> SMADLLVPKLTASVTDGAVGVTVDAPVSVTAADGVLAAVTMVNDNGRPVAGRLSPDGLRWSTTEQLGYNRRYTLNATALGLGGAATRQLTFQTSSPAHLTMPYVMPGDGEVVGVGEPVAIRFDENIADRGAAEKAIKITTNPPVEGAFYWLNNREVRWRPEHFWKPGTAVDVAVNTYGVDLGEGMFGEDNVQTHFTIG

The transpeptidase LtdMt2 catalyzes the formation of the (3–3) cross-links characteristic of the peptidoglycan layer in the Mycobacterium tuberculosis cell wall. The structure analysis reveals that LdtMt2 folds into three domains: two domains in the N-terminal part, both of which show an immunoglobulin-related fold, and a C-­terminal transpeptidase domain. Combining the structures of the two fragments provides a view of the complete three-domain extramembrane part of LdtMt2 and shows that the protein extends at least 80–100 Å from the plasma membrane into the peptidoglycan layer and thus defines the maximal distance at which cross-links are formed by this enzyme. LdtMt2 (Rv2518c) has been reported to be expressed at the highest level and has been found to be essential for virulence.

The structure of the AB-domain fragment, which was solved by molecular replacement to 1.45 Å resolution, reveals that despite a lack of overall sequence identity the A domain is structurally very similar to the B domain. The structure of the segment comprising the A and B domains was solved to 1.45 Å resolution by molecular replacement using the B domain (residues 149–250) as the search model. The structure of the AB module includes residues 57–250, approximately half of the extramembrane part of LdtMt2, and 309 water molecules. Each domain in the model contains a bound sulfate ion located on the protein surface. In domain A the sulfate is anchored to the protein through interactions with Asn95, Asn97, Arg99 and Arg122, whereas in the B domain the ligand forms hydrogen bonds to the side chains of Tyr201, Arg209 and Arg211. A structural classification of immunoglobulin-like β-­sandwich domains defined four subclasses, s-type, h-type, c-type and v-­type, based on strand connectivity and topology. Both immunoglobulin-like domains of LdtMt2 belong to the c-type Ig fold, with strand orders a–b–e–d and c–­f–g in the two antiparallel β-sheets. The similarity between the A and B domains is reflected in the Cα r.m.s.d. of 2.7 Å based on 85 aligned residues. The sequence identity derived from structural alignment of the two domains is 12% which does not provide strong evidence for gene duplication. The domain interface accounts for 350 Å2 of buried surface area including 13 and ten buried residues from the A and B domains, respectively. The domain interface is formed by the loops connecting β-strands β1 and β2 and β-­strands β5 and β6 in domain A and the loop connecting β-strands β6 and β7 in domain B. The two domains are connected by a short linker Ala149-His150 forming hydrogen bonds to the main chain of the B-­domain residues involved in the interface (Gly236 and Phe237).>MPPKQHRHQKKDKNDNALQNTIGFVPPGATLASVSGYRPPDAFVNRIDRNIPVPARLRHTPVSLIEAVNDFHYAMMNDEERNNFYYEVLKKHVTPETGVLEIGAGSGLLSLMAAKLGAKWVVAVEGSEELAKLARENIRANNMEHQVKVLHMMSTELKPKHLPEPPDVLLSEIFGTMMLGESALDYVVDVRNRLLKPTTKIIPQFGTQYAVPIECDALHRISSVSGWRDLDLKHMMTLQDTVSIVFAKHYGIRMNSVNFRRLSDPIELFRVDFSSSNRNDISRRKHFDVVAKESGTAHAMLFYWKVTDDEFVMSTDPEDTVNNFP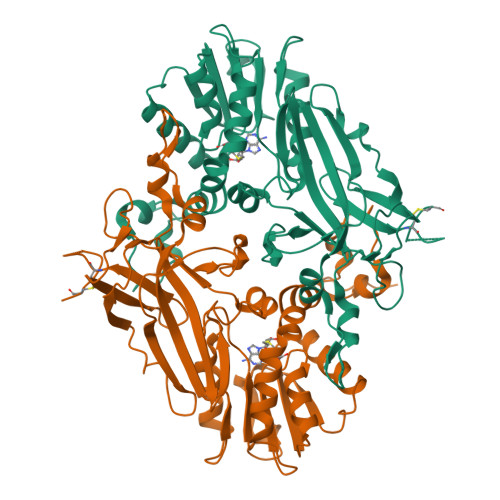RDMQWGQALQLLDASNGPLPTPVVFTEGKNYNFECNFSGDRVILHMQLCPESGNGEMTECEGKTT[2x]> SNAMPMTLDLQPGQRLARGVARHLRAHGFVSVEEFVPARGLRVDVMGLGPKGEIWVIECKSSRADFQADAKWQGYLEWCDRYFWAVDMEFPAELLPAESGLLIADAYDAEI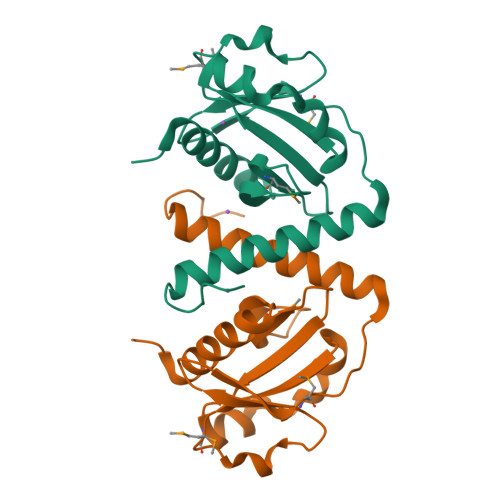VRMAPEQKLAPARRKVLIQKFATHAARRLQALRDPEGHGIFE>MSDTGLSFTPEKISTEIDFGTLSGKAKERVYLPEEKGRKASQLDWKYSNAPIVKGAFNWDLLPRVSVGASGWTTLAGRGGNMVDRDWLDTSNPGTWTDESKHPNTRLNFANEFDLNIKGWLLNQ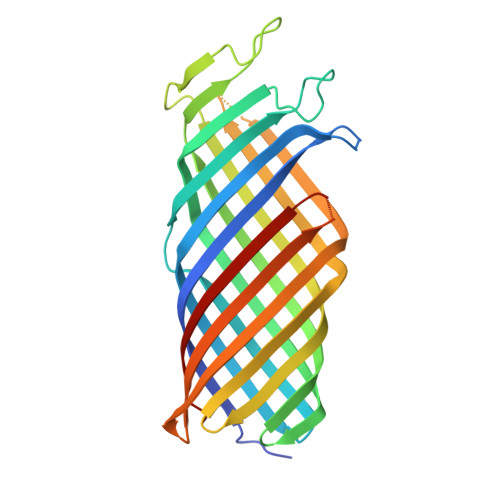PDYQLGLMAGYQENRYSFTAKGGSYIYSSEGGFRDETGSFPDGERAIGYKQHFKMPYIGLTGNYRYDSFEFGGSFKYSGWVKASDNDEHYNPEGRITYRSDVNNQNYYSVSLHAGYYITPAAKVYVEGTWNRITKKKGDTSLYSRNLNISDHTKNGAGIESYNFMTTAGLKYYF[2x]>[4x]SNAGMKFGEKSADILHRYPPMASIIDSG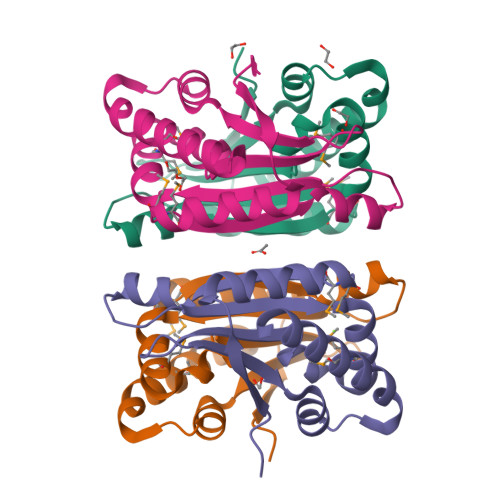LVTVESRHSVAETIERVAAKAKSMGMNVFTRVDHGAGAKEAGLGLPPTELIIFGNPQNGTVLMQDKRTIGLDLPIRALAWEDGSGKVWLTVNDPAWLAQRHSLGLSSDVAIKAMVTGTGTVTKYAAGD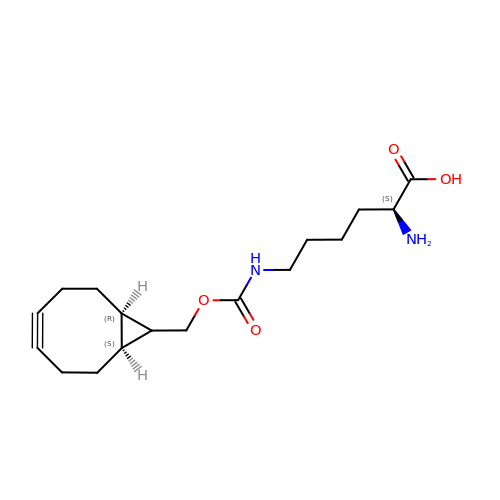N6-({[(1R,8S,9s)-bicyclo[6.1.0]non-4-yn-9-yl]methoxy}carbonyl)-L-lysine | C17 H26 N2 O4 | QLDVOCPEKYLEOT-XGUBFFRZSA-N(4R)-4-HYDROXY-N,N,N-TRIMETHYLPENTAN-1-AMINIUM | C8 H20 N O | 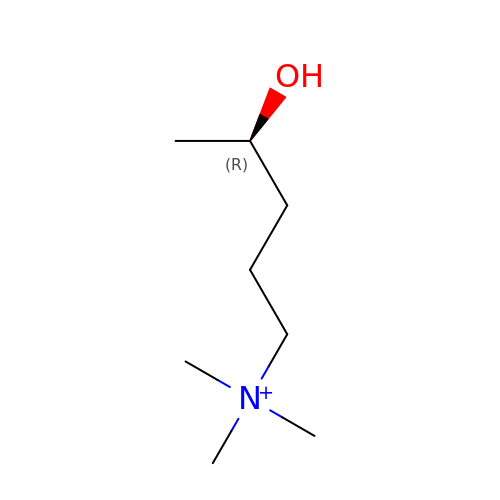HSBSNRZAOXKTSK-MRVPVSSYSA-N> MGSSHHHHHHSSGLVPRGSHNTRYNAADIEVLSGLDPVKRRPGMYTDTARPNHLAQEVIDNSVDEALAGHAKQIEVTLYKDGSCEVSDDGRGMPVDIHPEEKIPGVELILTRLHAGGKFNNRNYTFSGGLHGVGVSVVNALSTKVELFIKREGSEHRMEFRDGNAASKLEVVGTVGKKNTGTRLRFWADPKYFDTPKFNVRALRHLLRAKAVLCPGLTVKLHDEATGEQDSWYFENGLRDYLKGEMAEHEMLPADLFVGSLKKDTEIVDWAAGWVPEGELVQESYVNLIPTAQHGTHVNGLRSGLTDALREFCDFRNLLPRGVKLAP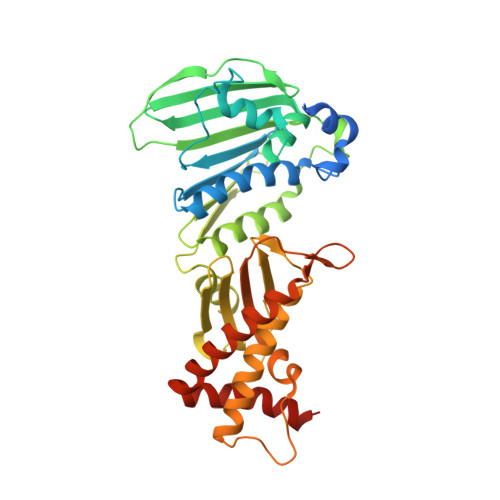EDVWDRVTFVLSLKMTDPQFSGQTKERLSSRQAAGFIEGAAHDAFSLYLNQNVEIGEKIAQIAIDRASARLKTEKQIVRKK>[2x]DPMKNTCKLLVVADHRFYRYMGRGEESTTTNYLIELIDRVDDIYRNTAWDNAGFKGYGIQIEQIRILKSPQEVKPGEKHYNMAKSYPNEEKDAWDVKMLLEQFSFDIAEEASKVCLAHLFTYQDFDMGTLGLAYVGSPRANSHGGVCPKAYYSPVGKKNIYLNSGLTSTKNYGKTILTKEADLVTTHELGHNFGAEHDPDGLAECAPNEDQGGKYVMYPIAVSGDHENNKMFSQCSKQSIYKT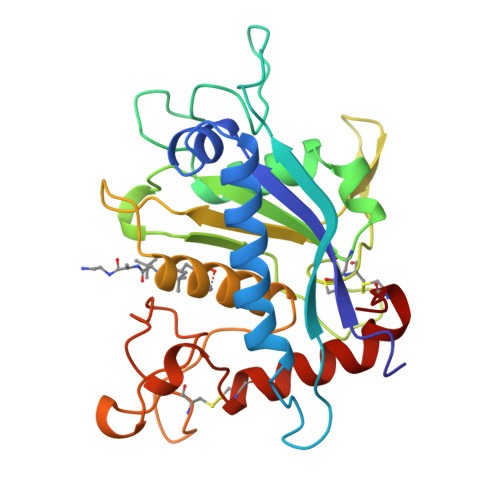IESKAQECFQERS;> DPMKNTCKLLVVADHRFYRYMGRGEESTTTNYLIELIDRVDDIYRNTAWDNAGFKGYGIQIEQIRILKSPQEVKPGEKHYNMAKSYPNEEKDAWDVKMLLEQFSFDIAEEASKVCLAHLFTYQDFDMGTLGLAYVGSPRANSHGGVCPKAYYSPVGKKNIYLNSGLTSTKNYGKTILTKEADLVTTHELGHNFGAEHDPDGKAECAPNEDQGGKYVMYPIAVSGDHENNKMFSQCSKQSIYKTIESKAQECFQERS;> DPMKNTCKLLVVADHRFYRYMGRGEESTTTNYLIELIDRVDDIYRNTAWDNAGFKGYGIQIEQIRILKSPQEVKPGEKHYNMAKSYPNEEKDAWDVKMLLEQFSFDIAEEASKVCLAHLFTYQDFDMGTLGLAYVGSPRANSHGGVCPKAYYSPVGKKNIYLNSGLTSTKNYGKTILTKEADLVTTHELGHNFGAEHDPDGLAECAPNEEQGGKYVMYPIAVSGDHENNKMFSQCSKQSIYKTIESKAQECFQERS We analysed a multidomain xylanase (Xyl) from the hindgut metagenome of the snouted harvester termite Trinervitermes trinervoides that releases xylobiose and xylotriose from beech and birch xylan and wheat arabinoxylan. The four domains of Xyl include an N-terminal GH11 xylanase domain, two family 36-like carbohydrate-binding domains CBM36-1 and 2, and a C-terminal CE4 esterase domain. Instead, individual domains and domain combinations were investigated structurally and for possible interdomain interactions. Xyl exemplifies a “beads-on-a-string” protein where the individual domains are “beads” each connected by a linker (string), with each domain retaining its individual function- making the synthesis of novel super enzymes for rapid and efficient degradation of bio-waste to biofuels within reach.

Xyl-CE4 at a concentration of 10 mg/mL in 20 mM Tris pH 7.5, 10 mM NaCl was crystallised in 8% (w/v) PEG 4000. The Xyl-CE4 domain encompasses 201 amino acid residues folded into eight α-helices, four β-strands and several extended loops that together create a distorted (α/β)-fold in which the β-strands form a curved inner β-sheet surrounded by the α-helices. The electron density of Xyl-CE4 reveals a metal ion bound through a distorted octahedral coordination by His643, His647, Asp593, a water molecule and an acetate ion. A single metal binding site identified in the crystal structure of Xyl-CE4 was correspondingly interpreted as Co2+ without further corroboration. EDTA treatment reduced enzyme activity to 0% of the untreated sample (0.2 μg Xyl-CE4 in 50 mM Tris pH 8.0). Addition of 10 mM Co2+, Mg2+ and Cu2+ restored the enzyme activity to 133, 122 and 110% of the original activity, respectively. Zn2+, the optimal ion for most CE4 enzymes, decreased the activity of Xyl-CE4 emphasizing the importance of identifying the optimal metal ions for each metalloenzyme. The esterase activity of Xyl-CE4 was investigated spectrophotometrically by monitoring the release of para-nitrophenol (p-NP) from 200 μL of 0.5 mM p-NPA at 405 nm and 30°C. Xyl-CE4 was active between pH 6.5 and 8.5 with maximum activity at pH 7.5. Catalytic activity of Xyl-CE4 between 20 and 80°C indicated a temperature optimum of 45°C. CD spectra recorded between 20 and 80°C yielded a melting temperature of 56°C.

> GNEKLIALTFDDGPSSTTSDVLDILERYGVKATFFLIGQNVNSNTLSIMQRQVRMGCELASHSYTHQDMTNMSAQNIRNEMEWTSSAIKNSVGVDVKFFRPPYIAVNNTMYQNIDYPFIQGTLINDSENSTSVQQRVNNALGAAKDGQIILLHDFQGNSQTVQALPQIIEGLKNQGYTFVTVSELFEKKGVNPNVEYKIWSNANGQHHHHHH> MSSAATVDPNEAFGLITKNLQEVLNPQIIKDVLEVQKRHLKLYWGTAPTGRPHCGYFVPMTKLADFLKAGCEVTVLLADLHAFLDNMKAPLEVVNYRAKYYELTIKAILRSINVPIEKLKFVVGSSYQLTPDYTMDIFRLSNIVSQND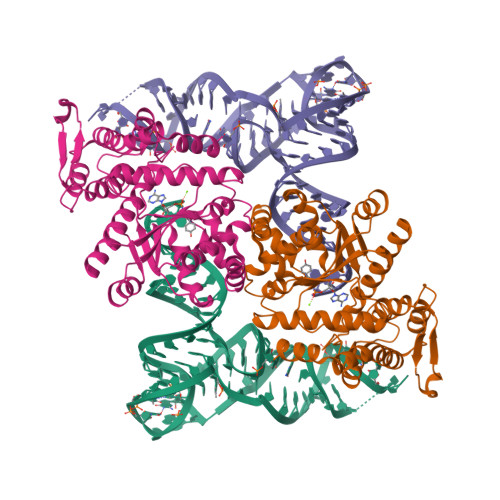AKRAGADVVKQVANPLLSGLIYPLMQALDEQFLDVDCQFGGVDQRKIFVLAEENLPSLGYKKRAHLMNPMVPGLAQGGKMSASDPNSKIDLLEEPKQVKKKINSAFCSPGNVEENGLLSFVQYVIAPIQELKFGTNHFEFFIDRPEKFGGPITYKSFEEMKLAFKEEKLSPPDLKIGVADAINELLEPIRQEFANNKEFQEASEKGYPVATPQKSKKAKKPKNKGTKYPGATKTNEIATKLEETKL>[6x]GPSRATMDTESQYSGYSYKSGHSRSSRKHRDRRDRHRSKSRDGGRGDKSVTIQAPGEPLLDNESTRGDERDDNWGETTTVVTGTSEHSISHDDLTRIAKDMEDSVPLDCSRHLGVAAGATLALLSFLTPLAFLLLPPLLWREELEPCGTACEGLFISVAFKLLILLLGSWALFFRRPKASLPRVFVLRALLMVLVFLLVVSYWLFYGVRILDARERSYQGVVQFAVSLVDALLFVHYLAVVLLELRQLQPQFTLKVVRSTDGASRFYNVGHLSIQRVAVWILEKYYHDFPVYNPALLNLPKSVLAKKVSGFKVYSLGEENSTNNSTGQSRAVIAAAARRRDNSHNEYYYEEAEHERRVRKRRARLVVAVEEAFTHIKRLQEEEQKNPREVMDPREAAQAIFASMARAMQK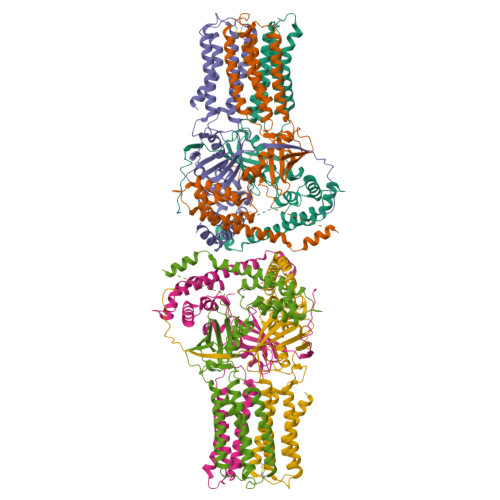YLRTTKQQPYHTMESILQHLEFCITHDMTPKAFLERYLAAGPTIQYHKERWLAKQWTLVSEEPVTNGLKDGIVFLLKRQDFSLVVSTKKVPFFKLSEEFVDPKSHKFVMRLQSETSV>[3x]AEIYNKDGNKVDLYGKAVGLHYFSKGNGENSYGGNGDMTYARLGFKGETQINSDLTGYGQWEYNFQGNNSEGADAQTGNKTRLAFAGLKYADVGSFDYGRNYGVVYDALGYTDMLPEFGGDTAYSDDFFVGRVGGVATYRNSNFFGLVDGLNFAVQYLGKNERDTARRSNGDGVGGSISYEYEGFGIVGAYGAADRTNLQEAQPLGNG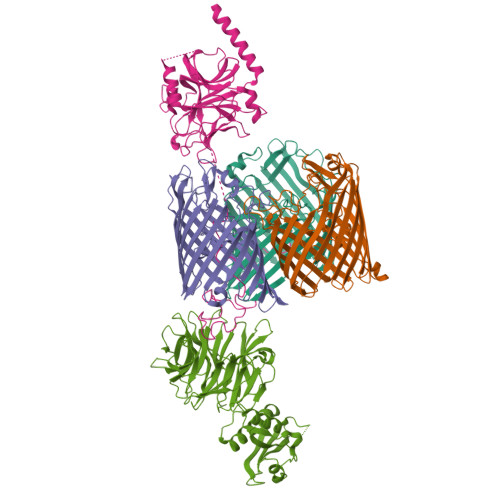KKAEQWATGLKYDANNIYLAANYGETRNATPITNKFTNTSGFANKTQDVLLVAQYQFDFGLRPSIAYTKSKAKDVEGIGDVDLVNYFEVGATYYFNKNMSTYVDYIINQIDSDNKLGVGSDDTVAVGIVYQF;> MSGGDGRGHNTGAHSTSGNINGGPTGIGVSGGCSDGSGWSSENNPWGGGSGSGIHWGGGSGRGNGGGNGNSGGGSGTGGNLSAVAAPVAFGFPALSTPGAGGLAVSISASELSAAIAGIIAKLKKVNLKFTPFGVVLSSLIPSEIAKDDPNMMSKIVTSLPADDITESPVSSLPLDKATVNVNVRVVDDVKDERQNISVVSGVPMSVPVVDAKPTERPGVFTASIPGAPVLNISVNDSTPAVQTLSPGVTNNTDKDVRPAGFTQGGNTRDAVIRFPKDSGHNAVYVSVSDVLSPDQVKQRQDEENRRQQEWDAT;> MKQALRVAFGFLILWASVLHAEVRIVIDSGVDSGRPIGVVPFQWAGPGAAPEDIGGIVAADLRNSGKFNPLDRARLPQQPGSAQEVQPAAWSALGIDAVVVGQVTPNPDGSYNVAYQLVDTGGAPGTVLAQNSYKVNKQWLRYAGHTASDEVFEKLTGIKGAFRTRIAYVVQTNGGQFPYELRVSDYDGYNQFVVHRSPQCLMSPAWSPDGSKLAYVTFESGRSALVIQTLANGAVRQVASFPRHNGAPAFSPDGSKLAFALSKTGSLNLYVMDLASGQIRQVTDGRSNNTEPTWFPDSQNLAFTSDQAGRPQVYKVNINGGAPQRITWEGSQNQDADVSSDGKFMVMVSSNGGQQHIAKQDLATGGVQVLSSTFLDETPSLAPNGTMVIYSSSQGMGSVLNLVSTDGRFKARLPATDGQVKFPAWSPYL The self-labeling protein tags (SLPs) HaloTag7, SNAP-tag, and CLIP-tag allow the covalent labeling of fusion proteins with synthetic molecules for applications in bioimaging and biotechnology. The three most popular SLPs are HaloTag7 (HT7),14 SNAP-tag (SNAP),15 and CLIP-tag (CLIP)16. To guide the selection of an SLP–substrate pair and provide guidelines for the design of substrates, we report a systematic and comparative study of the labeling kinetics and substrate specificities of HaloTag7, SNAP-tag, and CLIP-tag. We complement these kinetic studies by reporting crystal structures of HT7 and SNAP covalently labeled with rhodamine-based fluorophores, providing a detailed understanding of their substrate preferences.

SNAP was engineered from the human O6-alkylguanine-DNA alkyltransferase (hAGT), a protein involved in the repair of alkylated DNA by transferring alkyl moieties to its reactive cysteine. SNAP irreversibly transfers the benzyl moiety of the substrate to its reactive cysteine, leading to the release of guanine. The structure shows the same α/β topology with two domains as observed for hAGT and other SNAP structures. The TMR moiety strongly participates in the crystal packing, engaging in interactions with the neighboring xanthene ring and protein in a sandwichlike topology. As a consequence, and in contrast to HT7-TMR, SNAP does not interact with the bound fluorophore in the X-ray structure presented here. In the crystal structure of TMR-labeled SNAP, a structural ethylene glycol forms hydrogen bonds with both the backbone carbonyl oxygen of I31 and the carbonyl oxygen of the amide linking the benzyl to the fluorophore. This benzyl-fluorophore amide is also forming a hydrogen bond to the backbone carbonyl oxygen of residue E159 via its Nα atom. We modeled the SNAPf mutation E30R in the structure of TMR-labeled SNAP to gain a better understanding of how it affects the labeling kinetics. The results suggest that an arginine at position 30 could interact with the carbonyl oxygen of the amide group in the label via a moderate hydrogen bond (3.2 Å), replacing the hydrogen bond observed with the ethylene glycol in the crystal structure. This could lead to an increased affinity for the substrate or a better substrate positioning for labeling.

> GDCEMKRTTLDSPLGKLELSGCEQGLHEIIFLGKGTSAADAVEVPAPAAVLGGPEPLMQATAWLNAYFHQPEAIEEFPVPALHHPVFQQESFTRQVLWKLLKVVKFGEVISYSHLAALAGNPAATAAVKTALSGNPVPILIPCHRVVQGDLDVGGYEGGLAVKEWLLAHEGHRLGKR(5R)-5-[2-(4-methoxyphenyl)ethyl]-5-methylimidazolidine-2,4-dione 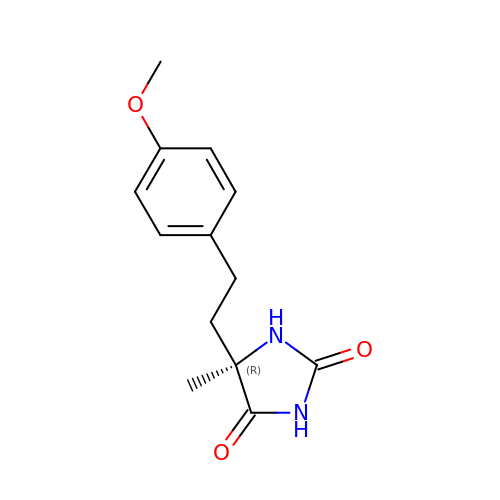| C13 H16 N2 O3 | HYRDVXQOZUFAFW-CYBMUJFWSA-N> LVHVASVEKGRSYEDFQKVYNAIALKLREDDEYDNYIGYGPVLVRLAWHISGTWDKHDNTGGSYGGTYRFKKEFNDPSNA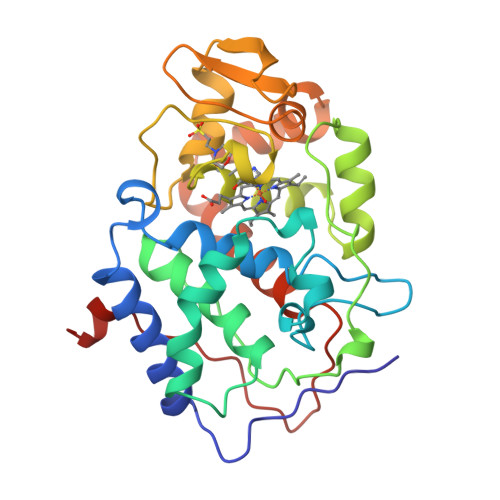GLQNGFKFLEPIHKEFPWISSGDLFSLGGVTAVQEMQGPKIPWRCGRVDTPEDTTPDNGRLPDADKDAGYVRTFFQRLNMNDREVVALMGAHALGKTHLKNSGYEGPYGAANNVFTNEFYLNLLNEDWKLEKNDANNEQWDSKSGYMMLPTDYSLIQDPKYLSIVKEYANDQDKFFKDFSKAFEKLLEDGITFPKDAPSPFIFKTLEEQGL> MSLPTFFLAPPLTEPFRARHRRKCIEKKDTFFQCLDKNKNETEPCEVEASGYSQ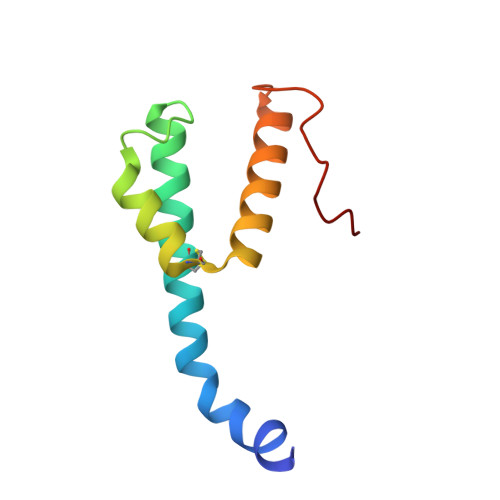ECPDSWRRYFNEQRWKALELKGEVKHANLKNTQQHF>IREILKMGDERLLRIAQPVPSELLGSEELQRLIDDMFETMHHVGGVGLAAPQIGVDLQLVIFGFERSERYPDAPAVPPTILLNPRITPLDDEMEEGWEGCLSVPGLRGAVSRHRRIRYQGLDPQGQPIDRSVEGFHARVVQHECDHLIGRLYPSRITDFSKFGFTE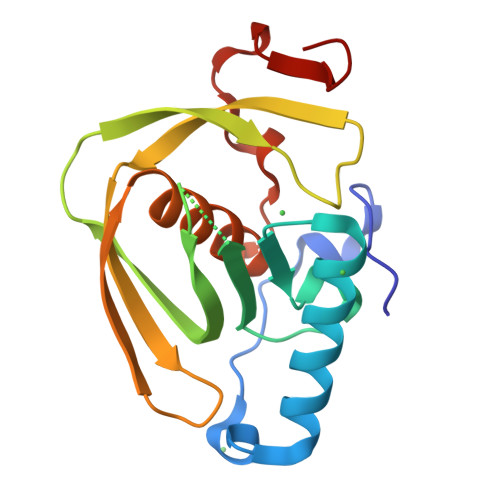VL[2x]In the present work, we focus on a class of monocyclic disulfide‐containing 19 amino acid peptides targeting the Vascular Endothelial Growth Factor‐A, the main pro‐angiogenic factor in Human. We proposed to use this peptide as a model to rationalize the thermodynamics of α‐helix stabilization by an i to i+4 lactam bridge. Around 950 Å2 of accessible surface area (ASA) was buried at the peptide‐VEGF interface, that overlapped with the VEGF receptor 1 domain 2 (VEGFR1‐d2)‐binding site. Although only lactam‐bridged ExxxK, DxxxK and KxxxD induced the formation of stable helix in the unbound state, all peptides of the series were helically folded when bound to VEGF.

Constraints caused by the lactam bridges and by the binding of the macro‐cyclized peptide to the VEGF site also made the α‐helices non‐canonical: in each of the four peptides, the residues P8‐11 folded into a 310‐helix characterized by a H‐bond between Glu P8 O and Cys P11 HN. For the peptides 1 c and 2 c (KxxxD and DxxxK), the DSSP software identified residues P9‐14 as an α‐helix, although Trp P9 O could bind to both Phe P12 HN and Glu P13 HN. The helix of peptide 4 c (KxxxE) was longer (residues P8 to P14) with a H‐bond network similar to peptide 2 c. In peptide 1 c, we also observed that the conformation of the lactam was compatible with a n→π* stabilizing interaction involving the linker amide carbonyl π* orbital and the Lys P10 main chain carbonyl n orbital, which was mentioned above. Interestingly the lactam bridge cyclization caused the side chains of residues P10 and P14 for peptide 1 c and 3 c to be in a non standard rotamer conformation, the consequence of which was moderate steric clashes involving hydrogen atoms. Therefore, lactam cyclization can result in sub‐optimal geometry with remaining steric constraints, where the side chains did not adopt the standard conformers (1 c and 3 c peptides). The real space correlation coefficient (RSCC) of the α‐helix was higher than 0.83 on VEGF:1 c, VEGF:2 c and VEGF:3 c structures, which supported these models. At this value, 1 c had 6 clusters, showing a larger flexibility in this segment than 2 c and 3 c, whereas 4 c and the monocyclic peptides had between 9 and 16 clusters. Bicyclic peptides 1 c, 2 c and 3 c had higher [θ]215 than the other peptides and ratios closer to 1, indicating that their C‐terminal α‐helices were mostly structured in unbound form. It corresponded to the mean Gibbs free energy gain due to the pre‐organization of bicyclic peptides 1 c, 2 c and 3 c compared to monocyclic analogs.

> CDIHVLWEWKCFEDL;>[2x]EVVKFMDVYQRSYCHPIETLVDIFQEYPDEIEYIFKPSCVPLMRCGGCCNDEGLECVPTEESNITMQIMRIKPHQGQHIGEMSFLQHNKCECRPK>[2x]MIIVSGQLLRPQDIENWQIDQDLNPLLKEMIETPVQFDYHSIAELMFELKLRMNIVAAAKTLHKSGAKFATFLKTYGNTTYWRVSPEGALELKYRMPPSKAIRDIAENGPFYAFECATAIVIIYYLALIDTIGEDKFNASFDRIILYDWHYEKLPIYTETGHHFFLGDCLYFKNPEFDPQKAQWRGENVILLGEDKYFAHGLGILNGKQIIDK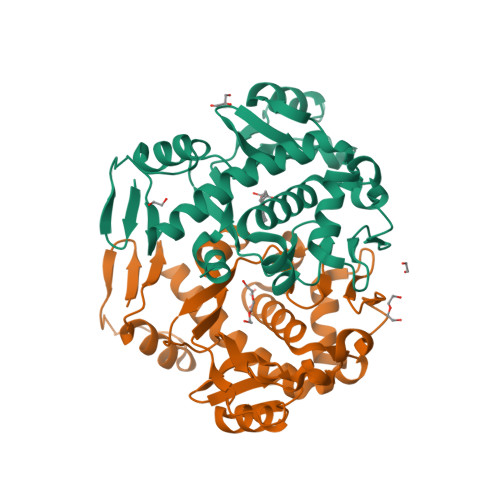LNSFRKKGALQSAYLLSQATRLDVPSLFRIVRVDKLAAALEHHHHHH>[4x]PGSIPLIGERFPEMEVTTDHGVIKLPDHYVSQGKWFVLFSHPADFTPVSTTEFVSFARRYEDFQRLGVDLIGLSVDSVFSHIKWKEWIERHI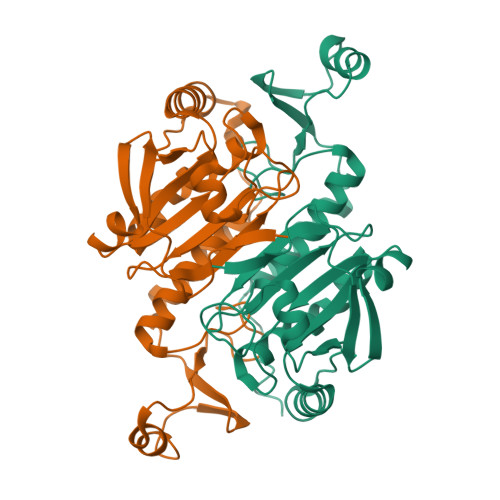GVRIPFPIIADPQGTVARRLGLLHAESATHTVRGVFIVDARGVIRTMLYYPMELGRLVDEILRIVKALKLGDSLKRAVPADWPNNEIIGEGLIVPPPTTEDQARARMESGQYRSLDAWFSWDTPASRDDVEEARRYLRRAAEKPAKLLYEEA>MEASAGMVAGSHKRNELVRIRHDSSDSGSKPLKSLNGQICQICGDTVGLTATGDVFVACNECAFPVCRPCYEYERKDGNQSCPQCKTRYKRHRGSPRVEGDEDEDDSDDIENEFNYAQGKAKARRQWEDDADLSSSSRRESQQPIPLLTNGQTMSGEIPCATPDTQSVRTTSGPLGPSEKVHSLPYVDPRQPVPVRIVDPSKDLNSYGLGNVDWKERVEGWKLKQEKNMVQMTGRYTEGKGGDVEGTGSNGEELQMVDDARQPMSRVVPIPSSQLTPYRVVIILRLIILGFFLQYRVTHPVKDAYPLWLTSVICEIWFALSWLLDQFPKWSPINRETYLERLALRYDREGEPSQLDPVDVFVSTVDPLKEPPLVTANTVLSILSVDYPVDKVSCYVSDDGSAMLTFEALSETAEFAKKWVPFCKKHNIEPRAPEFYFAQKIDYLKDKIQPSFVKERRAMKREYEEFKVRINALVAKAQKMPEEGWTMQDGTAWPGNNPRDHPGMIQVFLGHSGGLDTDGNELPRLVYVSREKRPGFQHHKKAGAMNALIRVSAVLTNGAYLLNVDCDHYFNNSKALKEAMCFMMDPVIGKKTCYVQFPQRFDGIDLHDRYANRNIVFFDINMKGQDGVQGP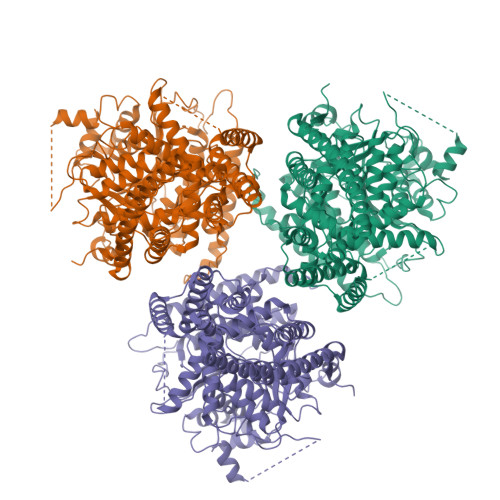VYVGTGCCFNRQALYGYDPVLTEEDLEPNIIVKSCWGSRKKGKGGNKKYSDKKKAMGRTESTVPIFNMEDIEEGVEGYDDERTLLMSQKSLEKRFGQSPVFIAATFMEQGGIPPSTNPATLLKEAIHVISCGYEDKTEWGKEIGWIYGSVTEDILTGFKMHARGWISIYCMPPRPAFKGSAPINLSDRLNQVLRWALGSIEIFLSRHCPLWYGYNGKLKPLMRLAYINTIVYPFTSIPLIAYCTLPAFCLLTNKFIIPEISNFASMWFILLFVSIFTTSILELRWSGVSIEDWWRNEQFWVIGGTSAHLFAVFQGLLKVLAGIDTNFTVTSKASDEDGDFAELYVFKWTSLLIPPTTVLIVNLVGIVAGVSYAINSGYQSWGPLFGKLFFAIWVIAHLYPFLKGLLGRQNRTPTIVIVWSVLLASIFSLLWVRIDPFTSDSNKLTNGQCGINC[3x]>ARLNITFSPQAFEDYKYFQQNNKKMVKKINELLKSIDRNGALEGIGKPEKLKSNLTGYYSRRINHEHRLVYTVDDNH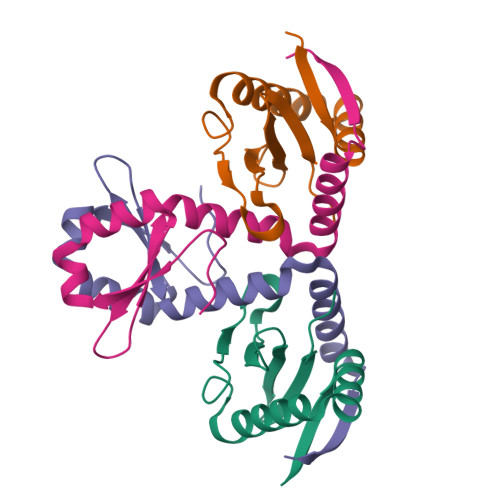IKIASCKYHY[2x];> SGLVPRGSHMIIKNYSYARQNLKALMTKVNDDSDMVTVTSTDDKNVVIMSESDYNSMMETLYLQQNPNNAEHLAQSIADLERGKTITKDIDV;> GLVPRGSHMIIKNYSYARQNLKALMTKVNDDSDMVTVTSTDDKNVVIMSESDYNSMMETLYLQQNPNNAEHLAQSIADLERGKTITKDIDV>[2x]GST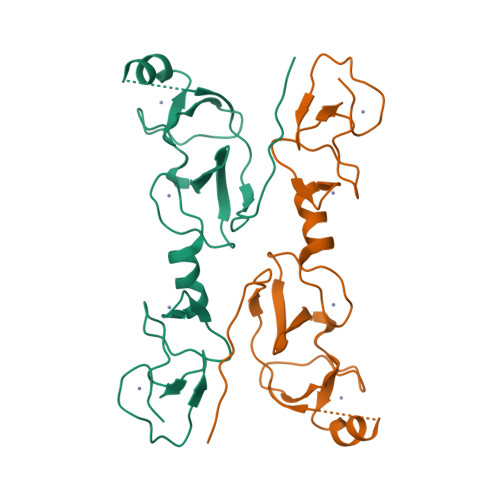PEIPMCAGCDQHILDRFILKALDRHWHSKCLKCSDCHVPLAERCFSRGESVYCKDDFFKRFGTKCAACQLGIPPTQVVRRAQDFVYHLHCFACVVCKRQLATGDEFYLMEDSRLVCKADYETAKQGGSGGSGGSGGGTPMVAASPERHDGGLQANPVEVQSYQPPW>MAVTNEEIKTASKIVRRVSNVEAFDKSGSVFKGYQIWTDISPTIENDPNIMFVKCVVQQGSKKEKLTVVQIDPPGTGTPYDIDPTHAWNCNSQVDPMSFGDIGLLNHTNIPCVLDFLKHRYLKNQIYTTAVPLIVAINPYKDLGN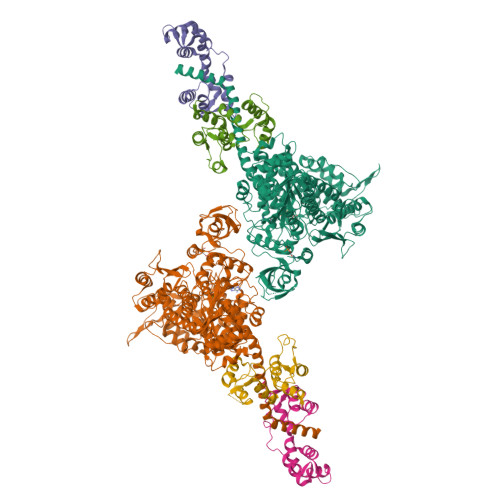TTNEWIRRYRDTADHTKLPPHVFTCAREALSNLHGVNKSQTIIVSGESGAGKTEATKQIMRYFASSKSGNMDLRIQTAIMAANPVLEAFGNAKTIRNNNSSRFGRFMQLVISHEGGIRYGSVVAFLLEKSRIITQDDNERSYHIFYQFLKGANSTMKSKFGLKGVTEYKLLNPNSTEVSGVDDVKDFEEVIESLKNMELSESDIEVIFSIVAGILTLGNVRLIEKQEAGLSDAAAIMDEDMGVFNKACELMYLDPELIKREILIKVTVAGGTKIEGRWNKNDAEVLKSSLCKAMYEKLFLWIIRHLNSRIEPEGGFKTFMGMLDIFGFEVFKNNSLEQLFINITNEMLQKNFVDIVFERESKLYKDEGISTAELKYTSNKEVINVLCEKGKSVLSYLEDQCLAPGGTDEKFVSSCATNLKENNKFTPAKVASNKNFIIQHTIGPIQYCAESFLLKNKDVLRGDLVEVIKDSPNPIVQQLFEGQVIEKGKIAKGSLIGSQFLNQLTSLMNLINSTEPHFIRCIKPNENKKPLEWCEPKILIQLHALSILEALVLRQLGYSYRRTFEEFLYQYKFVDIAAAEDSSVENQNKCVNILKLSGLSESMYKIGKSMVFLKQEGAKILTKIQREKLVEWENCVSVIEAAILKHKYKQKVNKNIPSLLRVQAHIRKKMVAQ[2x];>[2x]MKQECNVCYFNLPDPESTLGPYDNELNYFTWGPGFEYEPEPQRKPLSIEESFENSEESEESVADIQQLEEKVDESDVRIYFNEKSSGGKISIDNASYNARKLGLAPSSIDEKKIKELYGDNLTYEQYLEYLSICVHDKDNVEELIKMFAHFDNNCTGYLTKSQMKNILTTWGDALTDQEAIDALNAFSSEDNIDYKLFCEDILQ;> MASDMEEKFREAFILFSSCSDHIEMYKFFELMNSFGIILTNDEKAALPNDINMDYWLNFAKKHYNYEQPFKHINNVNEQNTNVQIKIDNFLGIMKALDTRLTESDLNILLQITNPENKTTLNLKTVSQKLTESI;> MASDMEEKFREAFILFSSCSDHIEMYKFFELMNSFGIILTNDEKAALPNDINMDYWLNFAKKHYNYEQPFKHINNVNEQNTNVQIKIDNFLGIMKALDTRLTESDLNILLQITNPENKSTLNLKTVSQKLTESI>NTLTVKMNDALSSGTGENIGEITVSETPYGLLFTPHLNGLTPGIHGFHVHTNPSCMPGMKDGKEVPALMAGGHLDPEKTGKHLGPYNDKGHLGDLPGLVVNADGTATYPLLAPRLKSLSELKGHSLMIHKGGDNYSDKP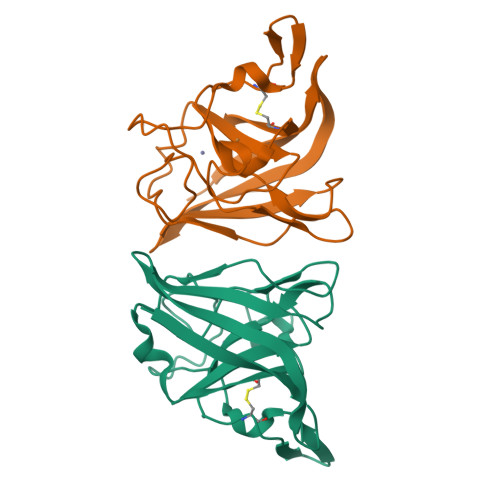APLGGGGARFACGVIEK[4x]> LA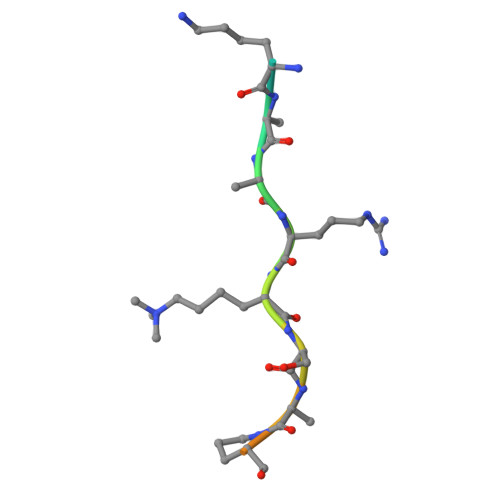TKAARKSAPATGGV Saf pili are often found in clinical isolates of Salmonella enterica. The saf operon is located on Salmonella enterica centisome seven genomic island, which consists of four contiguous genes encoding the major subunit (SafA), periplasmic chaperone (SafB), outer membrane usher (SafC) and minor subunit (SafD). Saf pili are assembled by the chaperone-usher (CU) secretion pathway. In the DSE step of Saf pili assembly, the N-terminal extension (Nte) of an incoming SafA replaces the chaperone G1 strand (in SafB) via a zip-in-zip-out mechanism, giving rise to a remarkable polymer of SafD-(SafA)n (n > 100).

In order to obtain soluble SafD, we engineered a self-complemented SafD-dsc, in which the N-terminal extension of SafA (i.e. the G strand) is fused with the C-terminus of SafD via an artificial DNKQ linker. The final model was refined to 2.2 Å resolution using program PHENIX.REFINE. The SafD-dsc structure reveals a classic immunoglobulin-like fold, in which A-G strands form a β-sandwich fold with two β sheets packed against each other. Using Dali server, SafD is predicted to belong to the Afa/Dr poly-adhesin subfamily containing DraD (r.m.s.d. of 1.5 Å for 134 Cα atoms), HdaB (1.6 Å for 143 Cα atoms), AfaD (2.5 Å for 142 Cα atoms), AafB (1.1 Å for 129 Cα atoms) and AggB (1.5 Å for 133 Cα atoms). Interestingly, SafD-dsc structure harbors one highly negative charged patch that could constitute the binding site of the unknown host receptor. Similar to the published SafA-ANte structure, the P1-P5 residues (i.e. Gln9, Lys11, Val13, Ile15 and Phe17) of donor G strand interacts directly with the hydrophobic groove in SafD. In SafD-dsc, a conserved Leu4 in SafANte was used to mimic Phe3, and the corresponding hydrophobic pocket is termed the P** pocket. The asymmetric unit (ASU) contains two SafD-dsc molecules. The superimposition of the SafD molecules shows interesting structural variations/flexibilities in LoopA-B on top of the P5 pocket. MD simulation of in PapD-PapGII complex suggested a regulatory role of LoopA-B. Based on these observations, it is reasonable to speculate that the Try13 sidechain of SafD might act as a molecular ‘switch’, regulating the access of incoming Nte peptide.

>AEKLQTTLRVGTYFRAGHVPDGMVLAQGWVTYHGSHSGFRVWSDEQKAGNTPTVLLLSGQQDPRHHIQVRLEGEGWQPDTVSGRGAILRTAADNASFSVVVDGNQEVPADTWTLDFKACALAQEDTDNKQGSFLPNSEQQKSVDIVFSS[2x]>GVHSFWDIAGPTARPVRLESLEDKRMAVDASIWIYQFLKAVRDQEGNAVKNSHITGFFRRICKLLYFGIRPVFVFDGGVPVLKRETIRQRKERRQGKRESAKSTARKLLANTTLSTSAERNVAENAFVEDELFEQQMKDKRDSDEVTMDMIKEVQELLSRFGIPYITAPMEAEAQCAELLQLNLVDGIITDDSDVFLFGGTKIYKNMFHEKNYVEFYDAESILKLLGLDRKNMIELAQLLGSDYTNGLKGMGPVSSIEVIAEFGNLKNFKDWYNNGQFDKRKQETENKFEKDLRKKLVNNEIILDDDFPSVMVYDAYMRPEVDHDTTPFVWGVPDLDMLRSFMKTQLGWPH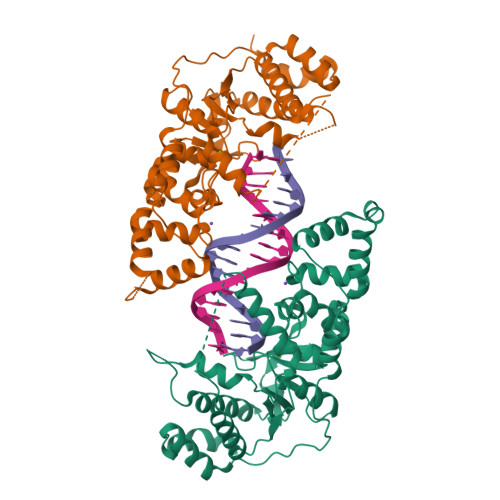EKSDEILIPLIRDV[2x]> TLQERLLAFERDRVTIPAAQVALAKQLAGDIALELQAYFRSKFPELPFGAFVPGGPLYDGLQAGAADHVRLLVPLVLEPGLWSLVPGVDTVARDPRCWAVRRTQLEFCPRGSSPWDRFLVGGYLSSRVLLELLRKALAASVNWPAIGSLLGCLIRPSMASEELLLEVQHERLELTVAVLVAVPGVDADDRLLLAWPLEGLAGNLWLQDLYPVEAARLRALDDHDAGTRRRLLLLLCAVCRGCSALGQLGRGHLTQVVLRLGEDNVDWTEEALGERFLQALELLIGSLEQASLPC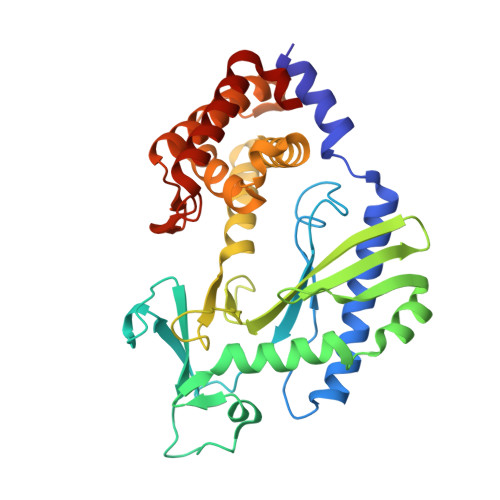HFNPSVNLFSSLREEEIDDIGYALYSGLQEPEGLL>[3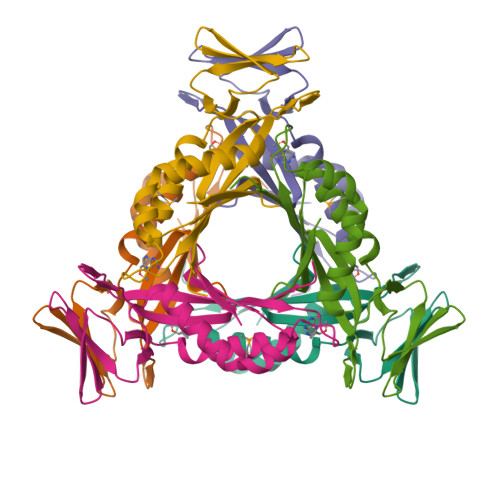x]MAHHHHHHMMKEETLNSDNSSAEVSVESPSFSFNCAHFIAYNGFRETLHGHNYNVSLKVRGYVRDDGYVIDFSILKEKVKKVCNKLDHHFILPIYSDVLKFENVKNNIKIICEDNSEYSFPERDCIKLPIKHSSTEEIGQYILNQLIEEMDVSLLKSRHIHYIEISVSESPTQKAIVHKYI>SNGLEDSSTISFITWNIDGLDGCNLPERARGVCSCLALYSPDVVFLQEVIPPYCAYLKKRAASYTIITGNEEGYFTAILLKKGRVKFKSQEIIPFPNTKMMRNLLCVNVSLGGNEFCLMTSHLESTREHSAERIRQLKTVLGKMQEAPDSTTVIFAGDTNLRDQEVIKCGGLPDNVFDAWEFLGKPKHCQYTWDTKANNNLRIPA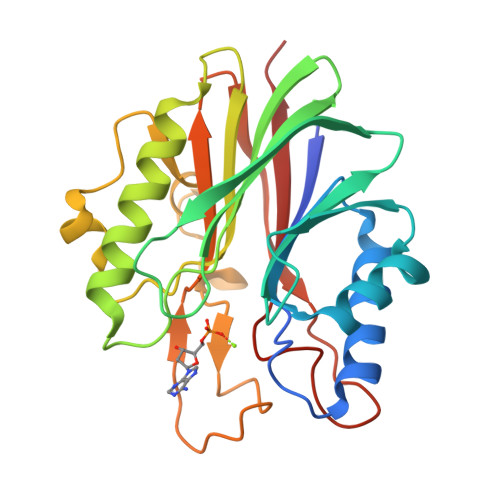AYKHRFDRIFFRAEEGHLIPQSLDLVGLEKLDCGRFPSDHWGLLCTLNVVL[9x]>SNAMADEIA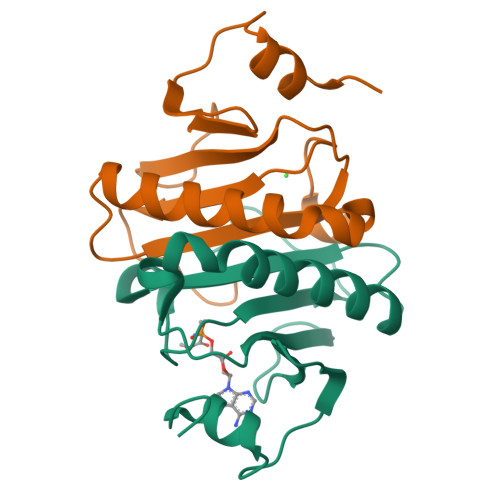KAQVARPGGDTIFGKIIRKEIPAKIIFEDDRCLAFHDISPQAPTHFLVIPKKHISQISVAEDDDESLLGHLMIVGKKCAADLGLNKGYRMVVNEGSDGGQSVYHVNLHVLGGRQMHWPPG[2x]>YGAPEPNVPSREALAVELSSQQEYLKLKERYDALQRTQRNLLGEDLGPLSTKELESLERQLDSSLKQIRALRTQFMLDQLNDLQSKERMLTETNKTLRLRLADG[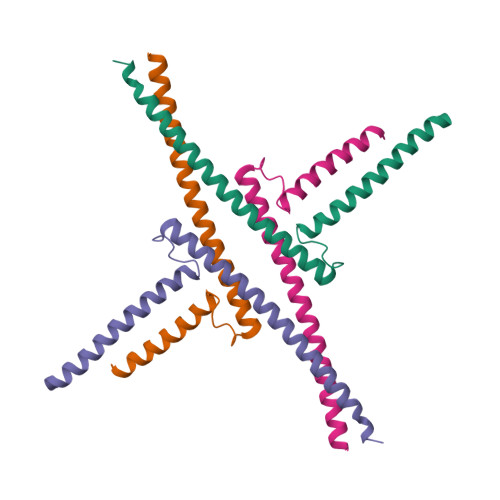4x]>GPLGSMSEEQVAQDTEEVFRSYVFYRHQQEQEAEGVAAPADPEMVTLPLQPSSTMGQVGRQLAIIGDDINRRYDSEFQTMLQHLQPTAENAYEYFTKIATSLFESGINWGRVVALLGFGYRLALHVYQHGLTGFLGQVTRFVVDFMLHHSIARWIAQRGGWVAALNLGNG[4x];>[4x]XSLLEKLAEELRQL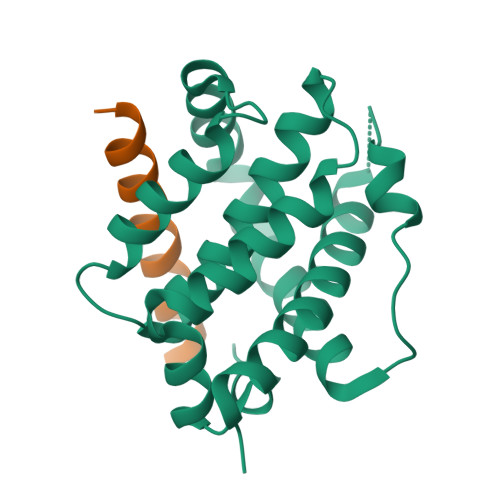ADELNKKFEKX> MYAIAFDLV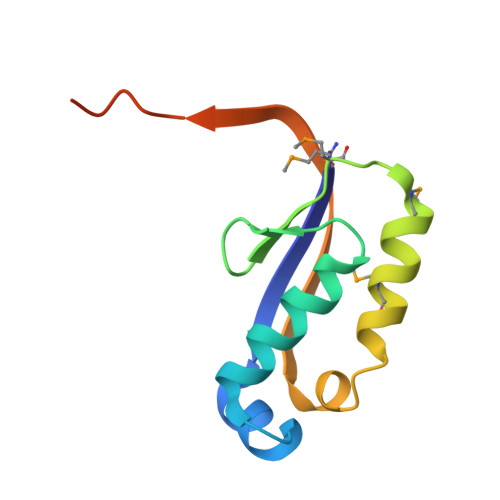VKDTQDYHPKGVQEAYTDIGAVLAKFGFVRTQGSLYTNMNEDMANLFQAMNALKQLAWISQSVRDIRAFRIEQWSDFTDFIRNLEHHHHHH> GHMKCRVWSEARVYTNINKQRTEEYWDYENTVIDWS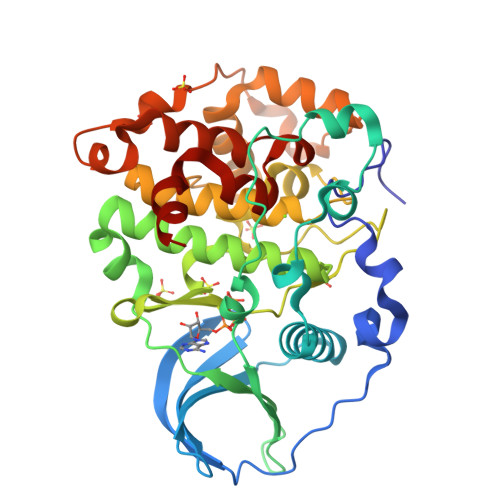TNTKDYEIENKVGRGKYSEVFQGVKLDSKVKIVIKMLKPVKKKKIKREIKILTDLSNEKVPPTTLPFQKDQYYTNQKEDVLKFIRPYIFDQPHNGHANIIHLFDIIKDPISKTPALVFEYVDNVDFRILYPKLTDLEIRFYMFELLKALDYCHSMGIMHRDVKPHNVMIDHKNKKLRLIDWGLAEFYHVNMEYNVRVASRFFKGPELLVDYRMYDYSLDLWSFGTMLASMIFKREPFFHGTSNTDQLVKIVKVLGTSDFEKYLLKYEITLPREFYDMDQYIRKPWHRFINDGNKHLSGNDEIIDLIDNLLRYDHQERLTAKEAMGHPWFAPIREQIEK> MGRGSERLPAVPSPTGTSVKSKNFRTVLYWQYPSMSETPHFVVEVKPYLSGKYQTVSTCVNISATSCDLSEEINEIFHSYWFRIKAIVGSQQSQYV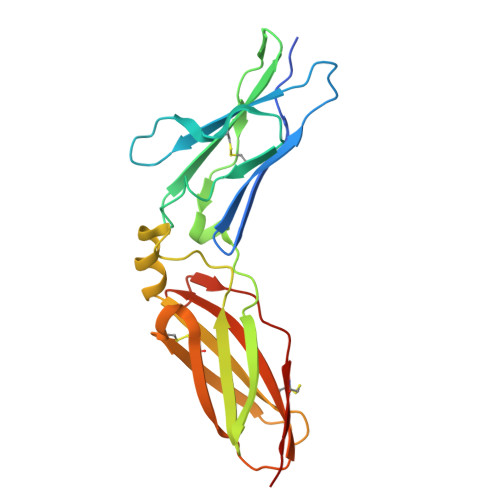ETDEFVLQKHGKIGPPKLNLSRHGAEIIVDVYHPEFPSVEVRPWMREIYSELSYSVIFRNSENESRKNFTVADCEMNECNLSIPVPSEGSTYCVSAKGHFFDDLIVGASSEESCIWVPITQA> GHMASGPWKLTASKTHIMKSADVEKLADELHMPSLPEMMFGDNVLRIQHGSGFGIEFNATDALRCVNNYQGMLK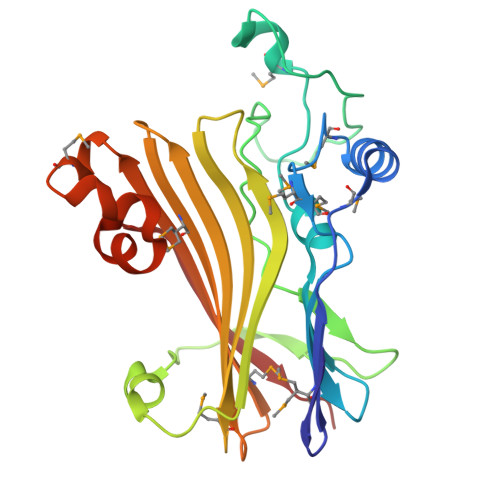VACAEEWQESRTEGEHSKEVIKPYDWTYTTDYKGTLLGESLKLKVVPTTDHIDTEKLKAREQIKFFEEVLLFEDELHDHGVSSLSVKIRVMPSSFFLLLRFFLRIDGVLIRMNDTRLYHEADKTYMLREYTSRESKISSLMHVPPSLFTEPNEISQYLPIKEAVCEKLIFPE> SAGINYVQNYNGNLGDFTYDESAG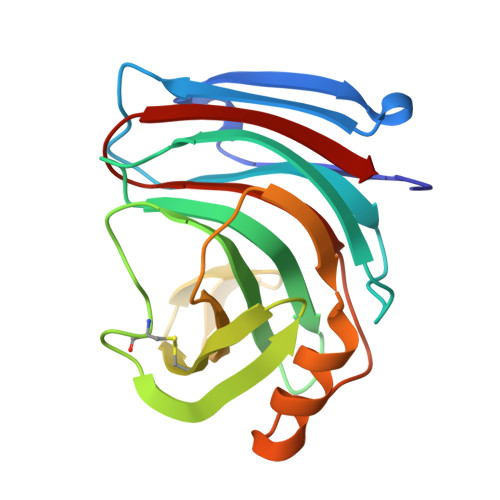TFSMYWEDGVSSDFVVGLGWTTGSSNAITYSAEYSASGSSSYLAVYGWVNYPQAEYYIVEDYGDYNPCSSATSLGTVYSDGSTYQVCTDTRTNEPSITGTSTFTQYFSVRESTRTSGTVTVANHFNFWAQHGFGNSDFNYQVMAVEAWSGAGSASVTISS>[2x]MTNSSASQKKRSKGSAQDWHRADIVAALHKRGITLAGLSRAHGL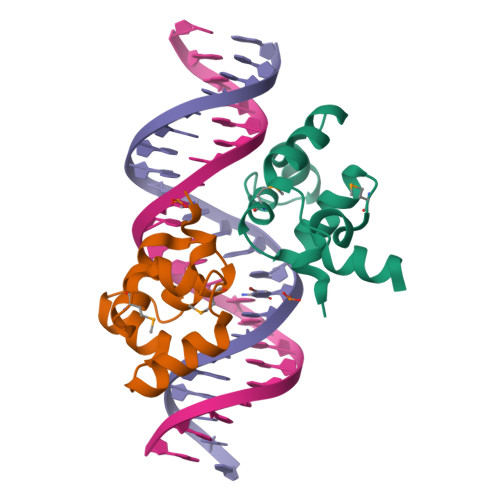AARTLSNAMERHYPRAERLIAQALDMRPEDIWPQRYRNKKTDGEKE The serine palmitoyltransferase (SPT) complex catalyzes the first and rate-limiting step in sphingolipid biosynthesis in all eukaryotes. ORM/ORMDL proteins are negative regulators of SPT that respond to cellular sphingolipid levels. We determined the cryo–electron microscopy structure of Arabidopsis SPT-ORM1 complex, composed of LCB1, LCB2a, SPTssa, and ORM1, in an inhibited state. The SPT-ORM1 complex is a ceramide sensor in the ER that controls cellular sphingolipid homeostasis.

All the variants, including ORM1-N17A, designed to weaken the coordination of ceramide polar head, and ORM1-S67R, ORM1-W20R, and ORM1-W88R, designed to repel ceramide aliphatic chains, exhibited greatly increased enzymatic activity compared to the wild-type (WT) SPT-ORM1 complex, supporting the importance of ceramide binding residues for ORM1-dependent SPT repression. The ORM1-N17A or ORM1-S67R mutation lowered the inhibitory potency of C6-phytoceramide, suggesting partially disrupted C6-phytoceramide binding. The overall structure of the ORM1-N17A variant is essentially identical to that of the WT SPT-ORM1 complex, except for two apparent local structural differences. As anticipated, the density corresponding to ceramide greatly diminished in the ORM1-N17A variant, confirming the largely disrupted ceramide binding by the mutation. The other evident structural difference is that the density corresponding to the ORM1 N terminus (residues 1 to 11, referred to as ORM1-N11) mostly disappeared without forming the hybrid β sheet in the ORM1-N17A variant, probably because of the flexible nature of the ORM1 N terminus in the absence of ceramide. The flexible ORM1 N terminus might not be able to suppress the acyl-CoA substrate entry efficiently, thus largely releasing the ORM1-dependent SPT inhibition at saturating substrate concentrations. Our results suggest that ceramide binding could induce the formation of a hybrid β sheet between the N termini of ORM1 and LCB2a, thus stabilizing the ORM1 N terminus in an inhibitory conformation that blocks substrate binding. The WT SPT-ORM1 complex represents a ceramide-bound state and has a decreased Vmax and an increased Khalf for palmitoyl-CoA compared to the ceramide-binding variant SPT-ORM1 (ORM1-N17A), indicating that the ceramide binding can repress SPT-ORM1 by mixed inhibition.

> PLTEQEIDELCDEWVPEPLIPPITEDMKHEPPVLESAAGPHTTVNGKDVVNFASANYLGLIGHEKLLESCTSALEKYGVGSCGPRGFYGTIDVHLDCETRISKFLGTPDSILYSYGLSTMFSTIPCFCKKGDVIVADEGVHWGIQNGLQLSRSTIVYFKHNDMESLRITLEKIMTKYKRSKNLRRYIVAEAVYQNSGQIAPLDEIVKLKEKYRFRVILDESNSFGVLGRSGRGLAEHHSVPIEKIDVVTAAMGHALATEGGFCTGNARIIDYQRLSSSGYVFSASLPPYLASAAITAIDVIDQNPDMLVKLKQNVALLWKGLSDIKGMSLTSNRESPIVFLKLEKSSGSAKDDLLLLEKMADRALKEDSLLVVSSKRSFLDKCRLPVGIKLYVSAGHSESDLLKASESLKRLASELLLKS;> MITIPYLTAVSTYFSYGLLFAFGQLRDFFRRFIDWWFTSNLQGYAPICLGHEDFYIRRLYHRIQDCFERPISSAPDAWFDVVERYSNDNNKTLKRTTKTSRCLNLGSYNYLGFGSFDEYCTPRVIESLKKFSASTCSSRVDAGTTSVHAELEECVTRFVGKPAAVVFGMGYATNSAIIPVLIGKGGLIISDSLNHSSIVNGARGSGATIRVFQHNTPSHLERVLREQIAEGQPRTHRPWKKIIVVVEGIYSMEGEICHLPEVVAICKKYKAYVYLDEAHSIGAIGKTGKGICELLGVDTADVDVMMGTFTKSFGSCGGYIAGSKELIQYLKHQCPAHLYATSIPTPSAQQIISAIKVILGEDGSNRGAQKLARIRENSNFFRAELQKMGFEVLGDNDSPVMPIMLYNPAKIPAFSRECLRQKVAVVVVGFPATPLLLARARICISASHSREDLIRALKVISKVGDLSGIKYFPAEPKKIEQSKNDIKLD;> MADYKDDDDKSGPDEVDASGRMNWVQRKIYLYNVTFGLYMLDWWERYLFNSLVVVLMWFVLYNGTRYFSELFQRHLT;> MANLYVKAVPPPDMNRATEWFMYPGVWTTYMLILFFGWLVVLSVSGCSPGMAWTVVNLAHFVVTYHSFHWMKGTPFADDQGIYNGLTWWEQMDNGQQLTRNRKFLTLVPVVLYLIASHTTDYRHPWLFLNTLAVMVLVVAKFPNMHKVRIFGINGDK;> MASNLVEMFNAALNWVTMILESPSARVVLFGVPIRGHFFVEGLLGVVIIILLTRKSYKPPKR>MSSVTWAPGNYPSTRRSDHVDTYQSASKGEVPVPDPYQWLEESTDEVDKWTTAQADLAQSYLDQNADIQKLAEKFRASRNYAKFSAPTLLDDGHWYWFYNRGLQSQSVLYRSKEPALPDFSKGDDNVGDVFFDPNVLAADGSAGMVLCKFSPDGKFFAYAVSHLGGDYSTIYVRSTSSPLSQASVAQGVDGRLSDEVKWFKFSTIIWTKDSKGFLYQRYPARERHEGTRSDRNAMMCYHKVGTTQEEDIIVYQDNEHPEWIYGADTSEDGKYLYLYQFKDTSKKNLLWVAELDEDGVKSGIHWRKVVNEYAADYNIITNHGSLVYIKTNLNAPQYKVITIDLSKDEPEIRDFIPEEKDAKLAQVNCANEEYFVAIYKRNVKDEIYLYSKAGVQLTRLAPDFVGAASIANRQKQTHFFLTLSGFNTPGTIARYDFTAPETQRFSILRTTKVNELDPDDFESTQVWYESKDGTKIPMFIVRHKSTKFDGTAAAIQYGYGGFATSADPFFSPIILTFLQTYGAIFAVPSIRGGGEFGEEWHKGGRRETKVNTFDDFIAAAQFLVKNKYAAPGKVAINGAANGGLLVMGSIVRAPEGTFGAAVPEGGVADLLKFHKFTGGQAWISEYGNPSIPEEFDY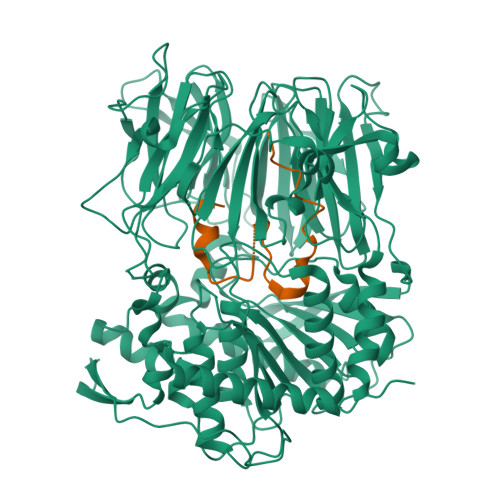IYPLSPVHNVRTDKVMPATLITVNIGDGRVVPMHSFKFIATLQHNVPQNPHPLLIKIDKSWLGHGMGKPTDKNVKDAADKWGFIARALGLELKTVE[4x];>MFDTNATRLPIWGIGCNPWTAEHVDQTLASGNDIC[4x]>SNAMKHYLICFDVQHDKTRAKLSRLLEKYGPRVQGSVFEVSFKTPDRKRQLEYKIHQIIKQSNTEENNIRFYNLNKDTIKHSHDINGNPIAQLPAAIVL[2x];>SNAMILPSFPDLTGLVVNLKFTARAEFSLNHEMAVDAFLRHSLNLGESYSHHLSIITPENGRLFYREGDTYRFVVIAMGNQQQTNSIWHTLINHLRKLPDSAPITDKQAPLRNNIKLESLNDLFDGIPVSSKESLDAYTLQRAMEQGLAWHKAANLTEQPLDIQWYWQSTVRILHADHKQHKGEQRYCRDAVQLTPLLLLKRIYETLNNVATYFGLKTNKNTTENHQAWLKEQAQYIEIQHPDLYWIDTPYFGKDAEKNTLGGMAGNFTLSLKPGIEPGLLAMLILTQMVGVGQRRTSGLGKYWLKHSLKHAHLILGLKPNRVTRSQTLLDCIIQPHIISQAIAEIEKKTNIDTLNERTLSQVQSAIGQLRKHQYQAPKLQGFTIPKKDGTERLLAVSPLYDRILQKAAAIVLTPGLDAIMSQASYGYRKGLSRQQVRYEIQNAYRQGYHWVYESDIEDFFDAVYRPQLINRLKSLLGNDPLWEQIESWLGQDIHIKDTIIERTPNLGLPQGSPLSPLLANFILDDFDSDLETHGFKIIRFADDFIILCKSQHEAQQAAHAVEQSLKEVKLSINVEKTHIIQLNQGFRFLGYLFREDHAIEIAGEKSDGRTTFAAEQTPTNLPPWLANLGTKSPQPLADDDLPKKSYGQIETQGTHLVLAGDAQIITTDNQNLIVKKDDKITHKISLEQLHAVTLIGLHTMTLPAKHRLLEHKIPVHIADRTGRYLGAVTSFQPAQNNYKNWFIQLQMCDREPFAHAIAQQIVISRIHNQRQTLLKRKAHRKQLQQTLSNLKKLQYKVTAATKRSSLNGLEGSATREYFQQFNLFLPEWAHFSKRTRRPPKDPFNVLLSLGYTILYSHTDAILQSAGFITWKGIYHQQSAAHAALASDIMESYRHLVERYAIYIINHGQIKQDDFRQEKDHLGQDTIRLSAEARRRYVGGLINRFQKFSKDKTLHQHLYQQAQQLKNAMHNQQSSQFQVWKELK[4x]

In some CRISPR systems, a reverse transcriptase (RT) fusion to the Cas1 integrase and Cas6 maturase creates a single protein that enables concerted sequence integration and crRNA production. In this work, we determine the 3.7 Å resolution structure of a naturally occurring Thiomicrospira Cas6-RT-Cas1—Cas2 complex using single particle cryo-electron microscopy (cryo-EM) and investigate its activities in vitro to elucidate how RT activity might coordinate with the CRISPR integrase and with the Cas6 maturation nuclease in the context of a Cas6-RT-Cas1 fusion protein. As observed for previous CRISPR integrase structures, the Cas6-RT-Cas1—Cas2 complex is heterohexameric, consisting of a central Cas2 dimer and two distal Cas6-RT-Cas1 dimers. In this study, we identify a type III Thiomicrospira Cas6-RT-Cas1—Cas2 complex containing three active sites for CRISPR spacer integration, reverse transcription, and RNA processing, and we observe all three activities in our reconstituted system.

The structure of the resulting Cas6-RT-Cas1—Cas2 complex was determined by single particle cryo-EM at an overall resolution of 3.7 Å. Approximately half of the complex displayed relatively lower local resolution, and refinement using a mask that excluded this region generated a reconstruction at 3.4 Å resolution with improved interpretability of high-resolution features. Portions of three Cas6-RT-Cas1 chains that were excluded by the mask were then rigid body docked and refined in the full complex reconstruction. The final model consists of two entire Cas2 chains, two entire Cas6-RT-Cas1 chains (excluding five poorly resolved loops), and the Cas1 domain from two additional Cas6-RT-Cas1 chains. Extending from the Cas1—Cas2 core are the Cas6-RT lobes, which are positioned orthogonal to the Cas1 domains relative to the central Cas2 dimer. The Cas6-RT lobe is connected to its associated Cas1 domain via a flexible linker, with the RT domain proximal to the central Cas2 dimer and the Cas6 domain closely abutting the RT domain. We observed density for the Cas6-RT lobe in two of the four Cas6-RT-Cas1 protomers (Cas1b and b’), presumably due to flexibility of the Cas6-RT domains in the other two Cas6-RT-Cas1 protomers (Cas1a and a’). No density was observed for the DNA substrate despite co-migration during size exclusion chromatography and indication of binding from electrophoretic mobility shift assays, suggesting that DNA was bound in only some of the complexes collected or that the DNA was lost during grid preparation or is too flexible to see. The most notable is an RT α-helix that serves as a direct connection between the RT and Cas1 active sites. While the N-terminal end of the RT-helix α9 is attached to the β-sheet containing the RT active site, the C-terminal end points into the catalytic Cas1a active site center.Bromodomains (BRDs) are protein interaction modules that specifically recognize ε-N-lysine acetylation motifs, a key event in the reading process of epigenetic marks. The 61 BRDs in the human genome cluster into eight families based on structure/sequence similarity. Despite large sequence variations, all BRD modules share a conserved fold that comprises a left-handed bundle of four α helices (αZ, αA, αB, αC), linked by loop regions of variable length (ZA and BC loops), which line the Kac binding site and determine binding specificity. The four helices form a deep cavity that is extended by the two loop regions (ZA and BC loops), creating a largely hydrophobic Kac binding pocket.

Interestingly, most of the 43 BRDs tested were highly sensitive to modifications flanking the Kac mark. Also, WDR9(2) and EP300 exclusively interacted with the triply modified H3 pT3K4acK9ac peptide.

>[12x]SMAPGQSKKKIFKPEELRQALMPTLEALYRQDPESLPFRQPVDPQLLGIPDYFDIVKSPMDLSTIKRKLDTGQYQEPWQYVDDIWLMFNNAWLYNRKTSRVYKYCSKLSEVFEQEIDPVMQSLG8-hydroxyquinoline-2-carboxylic 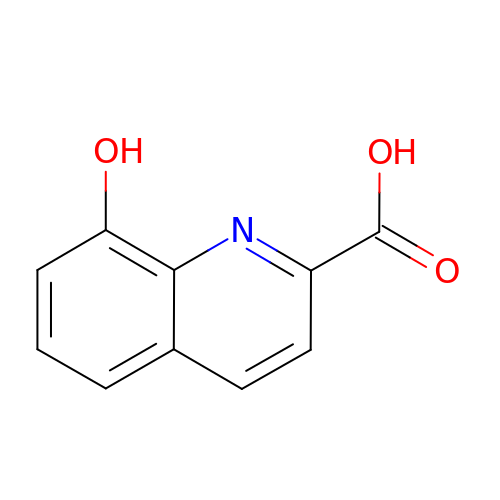acid | C10 H7 N O3 | UHBIKXOBLZWFKM-UHFFFAOYSA-N>MRVKAAQAGRQSSAKRHLAEQFAVGEIITDMAAAAWKVGLPIGQGGFGCIYLADMNSSESVGSDAPCVVKVEPSDNGPLFTELKFYQRAAKPEQIQKWIRTRKLKYLGVPKYWGSGLHDKNGKSYRFMIMDRFGSDLQKIYEANAKRFSRKTVLQLSLRILDILEYIHEHEYVHGDIKASNLLLNYKNPDQVYLVDYGLAYRYCPEGVHKAYAADPKRCHDGTIEFTSIDAHNGVAPSRRGDLEILGYCMIQWLTGHLPWEDNLKDPKYVRDSKIRYRENIASLMDKCFPAANAPGEIAKYMETVKLLDYTEKPLYENLRDILLQGLKAIGSKDDGKLDLSVVENGGLKAKTITKKRAAEIEE[4x]

Members of the Vaccinia-related kinase (VRK) family of serine/threonine protein kinases are present in the genomes of all metazoans and those of poxviruses, including the family-founding member vaccinia virus B1R1–6. Here we present the first crystal structures of the kinase domain of VRK1 and the first crystal structures for ligand-bound VRK1 and VRK2. Ligand-bound VRK kinase domains adopt the canonical protein kinase fold, except for the presence of the additional α-helix between αC and β4 (αC4) exclusively found on VRK proteins. The ligand-bound structures obtained here for active VRKs are in a closed, active conformation and display the same overall organization previously observed for the apo-structures, including the position of the VRK-exclusive αC4 and the structural organization of conserved residues that make up the kinase hydrophobic spine36.

For VRK13-364, 29 compounds displayed changes in melting temperatures, ΔTm, larger than 2.0 °C (an arbitrary cut off for a positive hit in this experiment), with the top hit, GW297361X, displaying a ΔTm of 9.7 °C. The VRK13-364/GW92761X structure has a less ordered N-terminal domain and in two of the crystal polypeptide chains (C and D) models start after the protein P-loop region (residues 68 or 80). Nevertheless, the most complete polypeptide chain in this model contains an intact P-loop (chain A, residues 22–341; used for the structural comparisons below). The crystal structures of VRK13-364/GW297361X (chain A) and VRK214-335/BI-D1870 reveal that the glycine-rich P-loop region of these kinases can adopt the so-called folded conformation. In the VRK13-364/GW297361X structure, the folded conformation of the P-loop is stabilized by a sulfur-π interaction between Phe48 and the sulfur atom in the thiazole moiety of GW297361X. Other than this interaction, VRK13-364 P-loop residues do not contact atoms in the compound. Ligand GW297361X can stabilize the protein N-lobe via a sulfur-π interaction with P-loop residue Phe48. In this position, the side chain of Phe48 approaches those of Asp197 in the DYG motif and Asn182 at the ATP-binding site entrance to create a hydrophobic tunnel over the compound. Another important interaction facilitated by GW297361X involves the sulfonamide group and residues located just outside the hinge region.> DVVVQAPTQVPGFLGDSVTLPCYLQVPNMEVTHVSQLTWARHGESGSMAVFHQTQGPSYSESKRLEFVAARLGAELRNASLRMFGLRVEDEGNYTCLFVTFPQGSRSVDIWLRVLAKPQNTAEVQKVQLTGEPVPMARCVSTGGRPPAQITWHSDLGGMPNTSQVPGFLSGTVTVTSLWILVPSSQVDGKNVTCKVEHESFEKPQLLTVNLTVYYPPEVSISGYDNNWYLGQNEATLTCDARSNPEPTGYNWSTTMGPLPPFAVA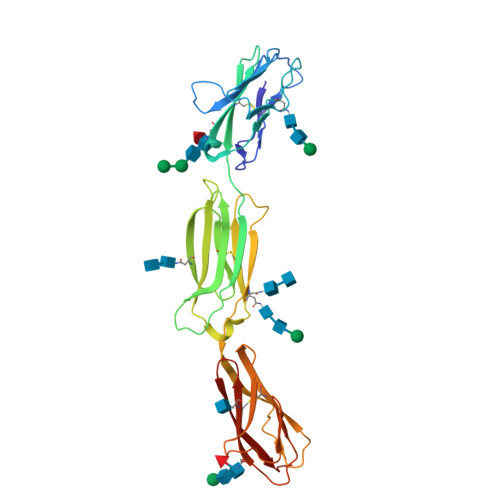QGAQLLIRPVDKPINTTLICNVTNALGARQAELTVQVKEGPPHHHHHH>MAKTVAYFYDPDVGNFHYGAGHPMKPHRLALTHSLVLHYGLYKKMIVFKPYQASQHDMCRFHSEDYIDFLQRVSPTNMQGFTKSLNAFNVGDDCPVFPGLFEFCSRYTGASLQGATQLNNKICDIAINWAGGLHHAKKFEASGFCYVNDIVIGILELLKYHPRVLYIDIDIHHGDGVQEAFYLTDRVMTVSFHKYGNYFFPGTGDMYEVGAESGRYYCLNVPLRDGIDDQSYKHLFQPVINQVVDFYQPTCIVLQCGADSLGCDRLGCFNLSIRGHGECVEYVKSFNIPLLVLGGGGYTVRNVARCWTYETSLLVEEAISEELPYSEYFEYFAPDFTLHPDVSTRIENQNSRQYLDQIRQTIFENL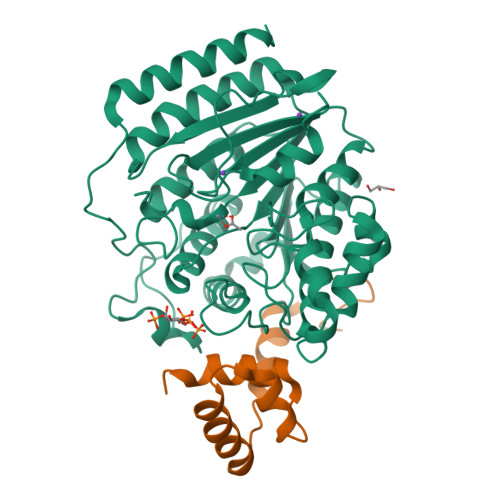KMLNHAPSVQ[2x];>GAMRQLAVIPPMLYDADQQRIKFINMNGLMADPMKVYKDRQVMNMWSEQEKETFREKFMQHPKNFGLIASFLERKTVAECVLYYYLTKKNENYK[2x]>[2x]GSHMHLTARGLTLDLSRPQVMGILNVTPDSFSDGGCHNNLDQALQHAQRMLSAGATLIDIGGESTRPGAAEVSEQEELDRVVPVVEALAQRFDVWLSVDTSKAAVITESAHAGAHLINDIRSLQEPGALEAAAKTGLPVCLMHMQGQPKNMQHSPYYDDLMTDINRFFQHHIERCVAAGIAKNKLLLDPGFGFGKNLAHNYQLLAHLSELHHFELPLLVGMSRKSMVGQLLNVPPQQRVIGSVACAVIAA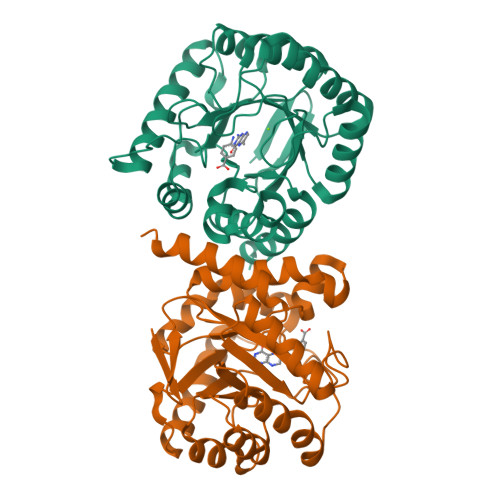MQGAQIIRVHDVKETVEAMCIVEATRSAKG>KCETIHVAIVCAGYNASRDVVTLVKSVLFHRRNPLHFHLIADSIAEQILATLFQTWMVPAVRVDFYNADELKSEVSWIPNKHYSGIYGLMKLVLTKTLPANLERVIVLDTDITFATDIAELWAVFHKFKGQQ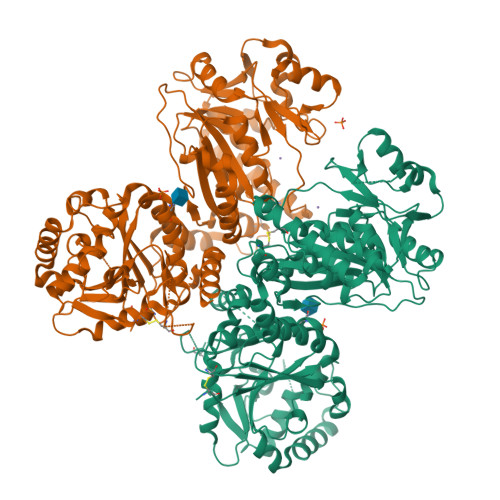VLGLVENQSDWYLGNLWKNHRPWPALGRGYNTGVILLLLDKLRKMKWEQMWRLTAERELMGMLSTSLADQDIFNAVIKQNPFLVYQLPCFWNVQLSDHTRSEQCYRDVSDLKVIHWNSPKKLRVKNKHVEFFRNLYLTFLEYDGNLLRRELFGCPSEADVNSENLQKQLSELDEDDLCYEFRRERFTVHRTHLYFLHYEYEPAADSTDVTLVAQLSMDRLQMLEAICKHWEGPISLALYLSDAEAQQFLRYAQGSEVLMSRHNVGYHIVYKEGQFYPVNLLRNVAMKHISTPYMFLSDIDFLPMYGLYEYLRKSVIQLDLANTKKAMIVPAFETLRYRLSFPKSKAELLSMLDMGTLFTFRYHVWTKGHAPTNFAKWRTATTPYRVEWEADFEPYVVVRRDCPEYDRRFVGFGWNKVAHIMELDVQEYEFIVLPNAYMIHMPHAPSFDITKFRSNKQYRICLKTLKEEFQQDMSRRYGFAALKYLTA[2x]> MPPQLHNGLDFSAKVIQGSLDSLPQEVRKFVEGNAQLCQPEYIHICDGSEEEYGRLLAHMQEEGVIRKLKKYDNCWLALTDPRDVARIASKTVIITQEQRDTVPIPKSGQSQLGRWMSEEDFEKAFNARFPGCMKGRTMYVIPFSMGPLGSPLAKIGIELTDSPYVVASMRIMTRMGTSVLEALGDGEFIKCLHSVGCPLPLKKPLVNNWACNPELTLIAHLPDRREIISFGSGYGGNSLLGKK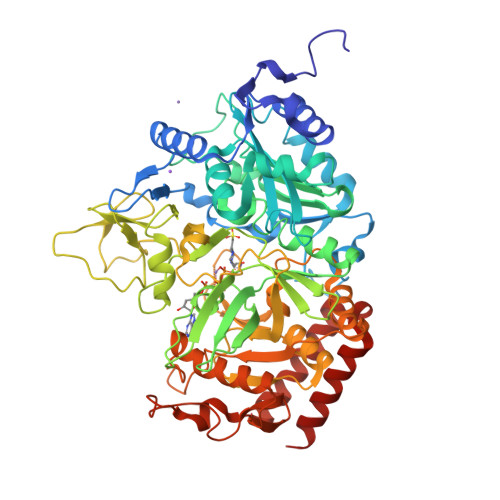CFALRIASRLAKEEGWLAEHMLILGITNPEGKKKYLAAAFPSACGKTNLAMMNPTLPGWKVECVGDDIAWMKFDAQGNLRAINPENGFFGVAPGTSVKTNPNAIKTIQKNTIFTNVAETSDGGVYWEGIDEPLAPGVTITSWKNKEWRPQDEEPCAHPNSRFCTPASQCPIIDPAWESPEGVPIEGIIFGGRRPAGVPLVYEALSWQHGVFVGAAMRSEATAAAEHKGKVIMHDPFAMRPFFGYNFGKYLAHWLSMAHRPAAKLPKIFHVNWFRKDKNGKFLWPGFGENSRVLEWMFGRIEGEDSAKLTPIGYVPKEDALNLKGLGDVNVEELFGISKEFWEKEVEEIDKYLEDQVNADLPYEIERELRALKQRISQM> GSMGCFFSKRRKADKESRPENEEERPKQYSWDQREKVDPKDYMFSGLKDETVGRLPGTVAGQQFLIQDCENCNIYIFDHSATVTIDDCTNCIIFLGPVKGSVFF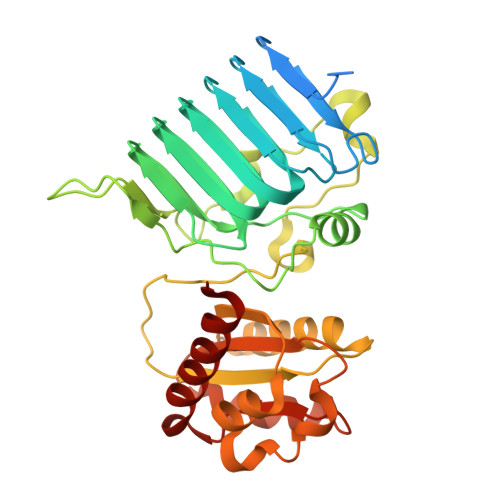RNCRDCKCTLACQQFRVRDCRKLEVFLCCATQPIIESSSNIKFGCFQWYYPELAFQFKDAGLSIFNNTWSNIHDFTPVSGELNWSLLPEDAVVQDYVPIPTTEELKAVRVSTEANRSIVPISRGQRQKSSDESCLVVLFAGDYTIANARKLIDEMVGKGFFLVQTKEVSMKAEDAQRVFREKAPDFLPLLNKGPVIALEFNGDGAVEVCQLIVNEIFNGTKMFVSESKETASGDVDSFYNFADIQMGI> MAKIAKTHEDIEAQIREIQGKKAALDEAQGVGLDSTGYYDQEIYGGSDSRFAGYVTSIAATELEDDDDDYSSSTSLLGQKKPGYHAPVALLNDIPQSTEQYDPFAEHRPPKIADREDEYKKHRRTMIISPERLDPFADGGKTPDPKMNARTYMDVMREQHLTKEEREIRQQLAEKAKAGELKVVNGAAASQPPSKRKRRWDQTADQTPGATPKKLSSWDQAETPGHTPSLRWDE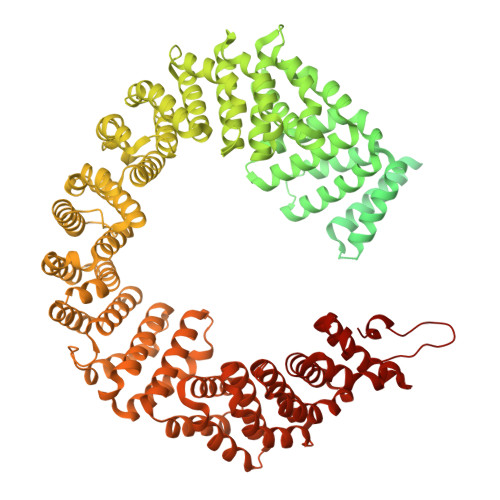TPGRAKGSETPGATPGSKIWDPTPSHTPAGAATPGRGDTPGHATPGHGGATSSARKNRWDETPKTERDTPGHGSGWAETPRTDRGGDSIGETPTPGASKRKSRWDETPASQMGGSTPVLTPGKTPIGTPAMNMATPTPGHIMSMTPEQLQAWRWEREIDERNRPLSDEELDAMFPEGYKVLPPPAGYVPIRTPARKLTATPTPLGGMTGFHMQTEDRTMKSVNDQPSGNLPFLKPDDIQYFDKLLVDVDESTLSPEEQKERKIMKLLLKIKNGTPPMRKAALRQITDKAREFGAGPLFNQILPLLMSPTLEDQERHLLVKVIDRILYKLDDLVRPYVHKILVVIEPLLIDEDYYARVEGREIISNLAKAAGLATMISTMRPDIDNMDEYVRNTTARAFAVVASALGIPSLLPFLKAVCKSKKSWQARHTGIKIVQQIAILMGCAILPHLRSLVEIIEHGLVDEQQKVRTISALAIAALAEAATPYGIESFDSVLKPLWKGIRQHRGKGLAAFLKAIGYLIPLMDAEYANYYTREVMLILIREFQSPDEEMKKIVLKVVKQCCGTDGVEANYIKTEILPPFFKHFWQHRMALDRRNYRQLVDTTVELANKVGAAEIISRIVDDLKDEAEQYRKMVMETIEKIMGNLGAADIDHKLEEQLIDGILYAFQEQTTEDSVMLNGFGTVVNALGKRVKPYLPQICGTVLWRLNNKSAKVRQQAADLISRTAVVMKTCQEEKLMGHLGVVLYEYLGEEYPEVLGSILGALKAIVNVIGMHKMTPPIKDLLPRLTPILKNRHEKVQENCIDLVGRIADRGAEYVSAREWMRICFELLELLKAHKKAIRRATVNTFGYIAKAIGPHDVLATLLNNLKVQERQNRVCTTVAIAIVAETCSPFTVLPALMNEYRVPELNVQNGVLKSLSFLFEYIGEMGKDYIYAVTPLLEDALMDRDLVHRQTASAVVQHMSLGVYGFGCEDSLNHLLNYVWPNVFETSPHVIQAVMGALEGLRVAIGPCRMLQYCLQGLFHPARKVRDVYWKIYNSIYIGSQDALIAHYPRIYNDDKNTYIRYELDYIL>GPHMFKSQTAILPEAGPFALYTLLKVRQNHAHVLQALKALPALVEEINQNQPGAELTVSVAFSKGFWSHFEMASPPELIDFPELGEGETHAPSTDVDVLIHCHATRHDLLFYTLRKGISDIAQDIEIVDETYGFRYLDARDMTGFIDGTENPKAEKRAEVALVADGDFAGGSYVMVQRFVHNLPAWNRLNLAAQEKVIGRTKPDSVELENVPAASHVGRVDIKEEGKGLKIVRHSLPYGSV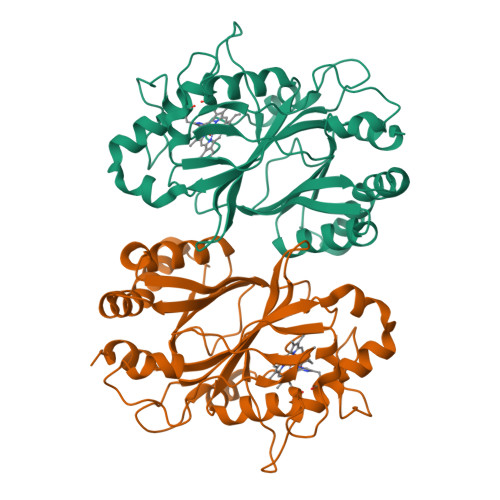SGDHGLLFIAYCHTLHNFKTMLESMYGVTDGKTDQLLRFTKAVTGAYFFAPSQVMLQELTLKNQ[4x]>[2x]MENNLENLTIGVFAKAAGVNVETIRFYQRKGLLL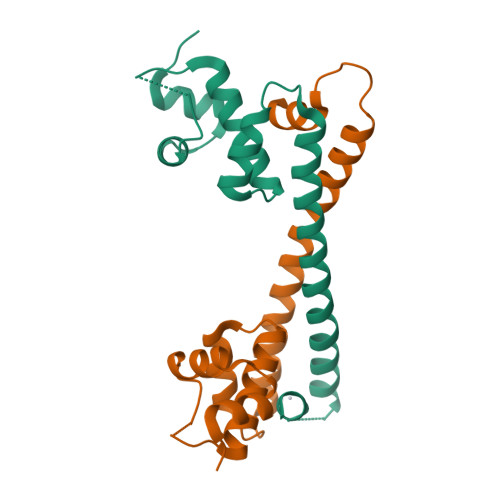EPDKPYGSIRRYGEADVTRVRFVKSAQRLGFSLDEIAELLRLEDGTHCEEASSLAEHKLKDVREKMADLARMEAVLSELVCACHARRGNVSCPLIASLQG> VVGGTEAQRNSWPSQISLQYRSGSSWAHTCGGTLIRQNWVMTAAHCVDRELTFRVVVGEHNLNQNDGTEQYVGVQKIVVHPYWNTDDVAAGYD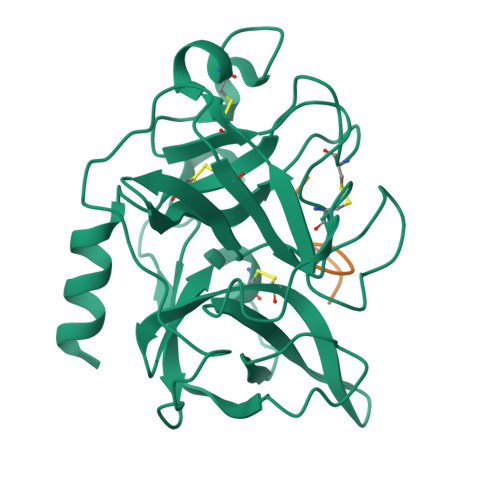IALLRLAQSVTLNSYVQLGVLPRAGTILANNSPCYITGWGLTRTNGQLAQTLQQAYLPTVDYAICSSSSYWGSTVKNSMVCAGGDGVRSGCQGDSGGPLHCLVNGQYAVHGVTSFVSRLGCNVTRKPTVFTRVSAYISWINNVIASN;> TTLKFPSDWDD>[4x]MKLSGGVEW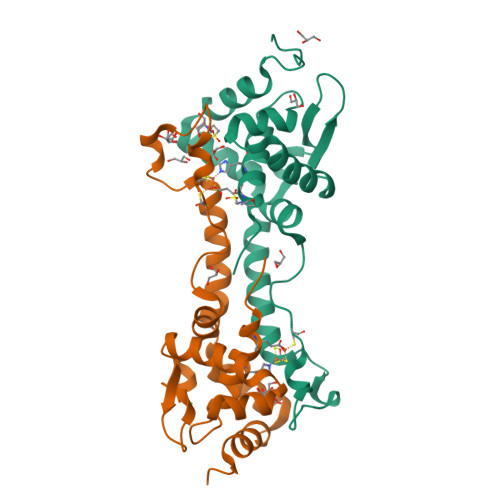ALHCCVVLTAASRPVPAARLAELHDVSPSYLAKQMQALSRAGLVRSVQGKTGGYVLTRPAVEITLLDVVQAVDGPDPAFVCTEIRQRGPLATPPEKCTKACPIARAMGAAEAAWRASLAATTIADLVATVDDESGPDALPGVGAWLIEGLGHHHHHH> MSDPFDYLFLEPLLIERIRSEVPGLAIVSGVPDLATLSEQDQPAPSAYVVYLGDE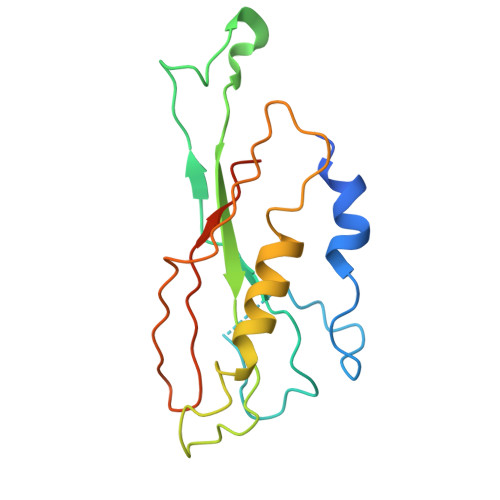TGTGADHQGGQRAIQTVGQQWAVVLVVHYADSSNSGEGARREAGPLLGRLVKALTGWAPAIDVAPLARSARQSPATYASGYLYFPLVFTARFVYPRIKSWKP>[2x]MRNDGGFLDWWEDLRSEMQSITD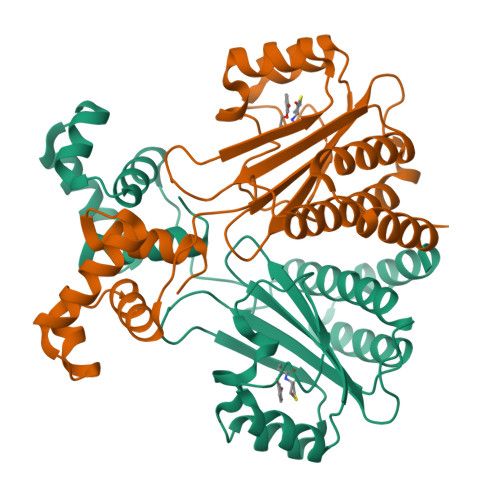SQEVFAVLEKEVRRLGFDYYAYCVRHPIPFTRPRIFMFGNYPPAWQEHYQAQNYFAIDPTIRHCLRSGNHIVWSDDLFADAQELWDDARDYGLRHGATHSCMAPNGVMGFLSVARSSPAISPHEREELRLRMRCLIELLHQTLTELNHPSLQSNPVCLSHREREILQWTADGKSSGEIAIILSISESTVNFHHKNIQKKFDAPNKTLAAAYAAALGLI N-Benzyl-2-methoxyacetamide 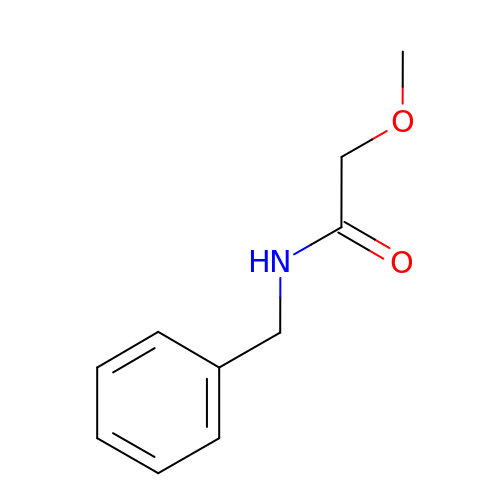| C10 H13 N O2 | VLAPGEODGZEQPC-UHFFFAOYSA-N> GPVDEIDKEVKKLEEEAKKSQEEVERLKQEVEKASKAGLDHEGDSRIFKK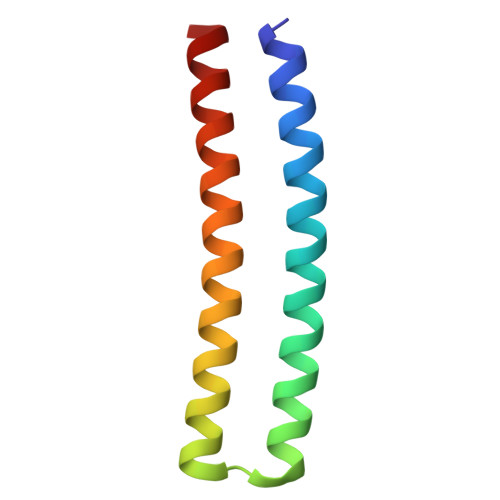IHDVVTKQIKVILRLIAVYAELVAIIG> STQTAEDKEEPLHSIISSTESVQGSTSKHEFQAETKKLLDIVARSLYSEKEVFIRELISNASDALEKLR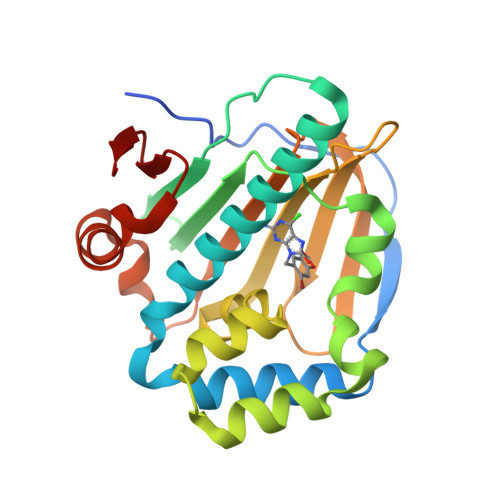HKLVSDGQALPEMEIHLQTNAEKGTITIQDTGIGMTQEELVSNLGTIARSGSKAFLDALQNQAEASSKIIGQFGVGFYSAFMVADRVEVYSRSAAPGSLGYQWLSDGSGVFEIAEASGVRTGTKIIIHLKSDCKEFSSEARVRDVVTKYSNFVSFPLYLNGRRMNT>[9x]MQRLFLLVAVMLLSGCLTAPPKEAARPTLMPRAQSYKDLTHLPAPTGKIFVSVYNIQDETGQFKPYPASNFSTAVPQSATAMLVTALKDSRWFIPLERQGLQNLLNERKIIRAAQENGTVAINNRIPLQSLTAANIMVEGSIIGYESNVKSGGVGARY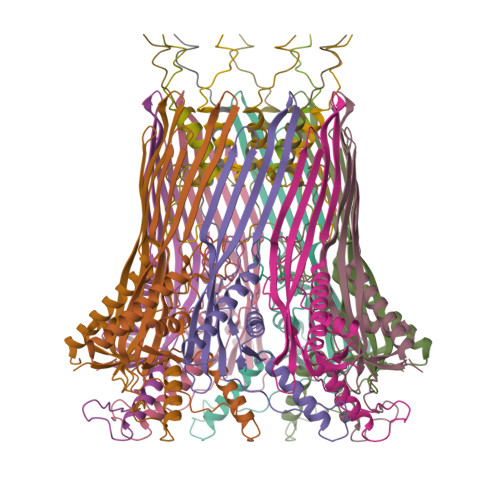FGIGADTQYQLDQIAVNLRVVNVSTGEILSSVNTSKTILSYEVQAGVFRFIDYQRLLEGEVGYTSNEPVMLCLMSAIETGVIFLINDGIDRGLWDLQNKAERQNDILVKYRHMSVPPESWSHPQFEK;>[9x]MRVKHAVVLLMLISPLSWAGTMTFQFRNPNFGGNPNNGAFLLNSAQAQNSYKDPSYNDDFGIETPSALDNFTQAIQSQILGGLLSNINTGKPGRMVTNDYIVDIANRDGQLQLNVTDRKTGQTSTIQVSGLQNNSTDFHHHHHH>GPGSNCGPPPTLSFAAPMDITLTETRFKTGTTLKYTCLPGYVRSHSTQTLTCNSDGEWVYNTFCIYKRCRHPGELRNGQVEIKTDLSFGSQIEFSCSEGFFLIGSTTSRCEVQDRGVGWSHPLPQCEI[2x];>[2x]GPGSESPREVTNELAASVWKKKVEEAKEKASKLEKQLEEAQKDYSEIEGKLEQFWHDYDKLEKENKEYASQLGKNQEEREKLELEYLRKSDEEYKEHQQYRQEQ

Antigenically sequence variable M proteins of the major bacterial pathogen Streptococcus pyogenes (Strep A) are responsible for recruiting human C4b-binding protein (C4BP) to the bacterial surface, which enables Strep A to evade destruction by the immune system. M proteins form parallel, dimeric α-helical coiled coils which are attached to the bacterial cell wall and extend ∼500 Å into the extracellular space. The most sequence divergent portion of M proteins, the hypervariable region (HVR), is responsible for binding C4BP. We identified C4BP-binding in several M proteins that lack an M2 or M22 pattern, and determined the structures of two, M68 and M87 protein HVRs, in complex with C4BPα1-2.

The structure of the complex between M87N100 and C4BPα1-2 was determined by molecular replacement to 2.7 Å resolution limit. The structure revealed the same global architecture observed previously, with two C4BPα1-2 molecules bound by dimeric, α-helical M87N100. The two M87 helices (aa 46–110 and 46–125) were asymmetric, with one less coiled than the other. Each C4BPα1-2 molecule contacted predominantly one of the two M87 helices, which we termed the “major” helix and the other the “minor” helix. The interface was dominated by negatively charged M protein amino acids interacting with positively charged C4BP ones, supplemented with a few hydrophobic contacts. The C4BPα2 quadrilateral as a whole was not involved in interaction, except for R64, which formed hydrophobic contacts using its aliphatic chain with M87 Y81 of the major helix and a salt bridge with D80 of the minor helix; Y81 was the only core a or d position amino acid involved in contacts. In contrast to the C4BPα2 quadrilateral, the C4BPα1 Arg39 nook had the same role as previously observed in the M2 pattern, forming hydrophobic contacts and a salt bridge to M protein. Here, the former was to M87 W92 of the major helix and the latter to D96 of the minor helix. Relative to WT M87 protein, Y81A, E89A, and D96A bound C4BP ∼21-fold less well on average, which indicated that the hydrophobic contact to C4BP R64 and polar contacts to K63 and R39, respectively, were crucial. With LL-37, the two M87 α-helices splay apart and no longer form a coiled coil in order to accommodate α-helical LL-37, which inserts between the two M87 helices, whereas with C4BP, the two M87 α-helices formed a coiled coil.>MAAALQTNIRTVKVPATFRAVSKQSLAPFRVRCAVASPGKKRYTITLLPGDGIGPEVVSIAKNVLQQAGSLEGVEFNFREMPIGGAALDLVGVPLPEETISAAKESDAVLLGAIGGYKWDNNEKHLRPEKGLLQIRAALKVFANLRPATVLPQLVDASTLKREVAEGVDLMVVRE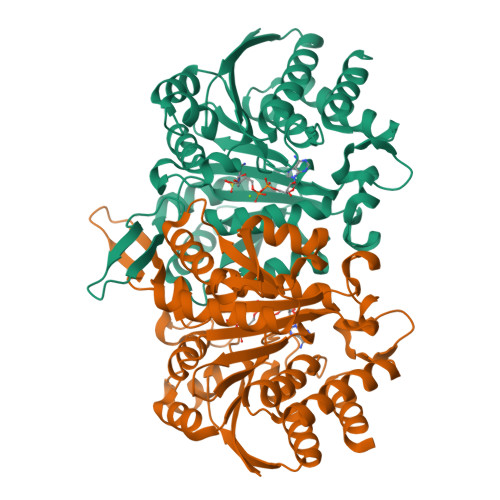LTGGIYFGEPRGIKTNENGEEVGFNTEVYAAHEIDRIARVAFETARKRRGKLCSVDKANVLEASILWRKRVTALASEYPDVELSHMYVDNAAMQLVRDPKQFDTIVTNNIFGDILSDEASMITGSIGMLPSASLSDSGPGLFEPIHGSAPDIAGQDKANPLATILSAAMLLKYGLGEEKAAKRIEDAVLVALNNGFRTGDIYSAGTKLVGCKEMGEEVLKSVDSQVPASV[8x]The insulin-related hormones regulate key life processes in Metazoa, from metabolism to growth, lifespan and aging, through an evolutionarily conserved insulin signalling axis (IIS). The dmIR primary structure, with ~33% sequence identity in the overlapping regions, suggests that its domain organisation is similar to human IR-like receptors. dmIR domain topology, similar to hIR, is made of unique (αβ)2 subunit homodimers, with the same modular, exons-reflecting organisation. We selected the Drosophila DILP5 for dmIR-ECD studies as a typical representative and well-characterised fly ILP, having also a high homology to human insulin (~28% sequence identity), and with nM-range KD for the dmIR high-affinity site 1 of 0.76 (±0.16) nM21 that is within a range of human insulin:hIR interaction (e.g., 0.2–0.7 nM). Here, we provide the 3-D description of an invertebrate IR-like receptor by determining the cryoEM structure of the dmIR-ECD in the complex with DILP5.

The 5:1 molar hormone:receptor ratio used for the preparation of the dmIR-ECD complex resulted in an asymmetric three-DILP5:dmIR-ECD arrangement. There are two adjacent insulins bound to sites 1 and 2’ on the down-arm/dynamic and static protomers, respectively, and one insulin at site 1’ on the arm-up/static protomer. The overall DILP5’s binding modes in site 1 (down-arm (Λ) and up-arm site 1’ (Γ)) follows closely engagements of human insulins in respective h(m)IR sites. However, the third DILP5 molecule binds to site 2’ on the FnIII-1’ domain of the static protomer being adjacent to - and in contacts with - the down-arm site 1-bound DILP5, while site 2 is unoccupied. However, DILP5 sits ~6 Å lower on the FnIII-1’ side-surface than insulin in hIR’s sites 2/2’, with its B-helix also closer by ~2.7 Å to the FnIII-1’, especially when compared at the Cα atoms of ValB16(LeuB17) (in brackets: corresponding sequences of hIR (or human insulin)). This lowering of site 2’ DILP5 is likely required for the simultaneous accommodation of both DILP5s in sites 1 and 2’ in the lower-arm environment. Here, the shorter Lys884-Gly886 FnIII-1 loop minimises the steric hindrance upon binding of both DILP5s into the lower arm site1/2’ space, while the longer – dmIR specific - Ala1168-Ser1189 loop (with central short Ile1173-Thr1181 helix) provides a supporting ledge for the site 2’-bound hormone. In the dmIR-ECD this loop is slightly longer, and—importantly—it is reconfigured into a narrow β-hairpin that points directly into the DILP5 binding cavity that would be occupied by the C-domain of single-chain insulin-like family of hormones. Another characteristic structural feature of the dmIR-ECD is the reshaped - and slightly longer than in the hIR - Ala594-615Asn (Cys259-280His) CR-domain loop, which may prevent binding of any insulin-like hormone with a significant C-domain (e.g., hIGF-1-like).

>[2x]MHNYSYSPGISLLLFILLANTLAIQAVVLPAHQQHLLHNDIADGLDKTALSVSGTQSRWTRSESNPTMRLSQNVKPCKSMDIRNMVSHFNQLENCTVIEGFLLIDLINDASPLNRSFPKLTEVTDYIIIYRVTGLHSLSKIFPNLSVIRGNKLFDGYALVVYSNFDLMDLGLHKLRSITRGGVRIEKNHKLCYDRTIDWLEILAENETQLVVLTENGKEKECRLSKCPGEIRIEEGHDTTAIEGELNASCQLHNNRRLCWNSKLCQTKCPEKCRNNCIDEHTCCSQDCLGGCVIDKNGNESCISCRNVSFNNICMDSCPKGYYQFDSRCVTANECITLTKFETNSVYSGIPYNGQCITHCPTGYQKSENKRMCEPCPGGKCDKECSSGLIDSLERAREFHGCTIITGTEPLTISIKRESGAHVMDELKYGLAAVHKIQSSLMVHLTYGLKSLKFFQSLTEISGDPPMDADKYALYVLDNRDLDELWGPNQTVFIRKGGVFFHFNPKLCVSTINQLLPMLASKPKFFEKSDVGADSNGNRGSCGTAVLNVTLQSVGANSAMLNVTTKVEIGEPQKPSNATIVFKDPRAFIGFVFYHMIDPYGNSTKSSDDPCDDRWKVSSPEKSGVMVLSNLIPYTNYSYYVRTMAISSELTNAESDVKNFRTNPGRPSKVTEVVATAISDSKINVTWSYLDKPYGVLTRYFIKAKLINRPTRNNNRDYCTEPLVKAMENDLPATTPTKKISDPLAGDCKCVEGSKKTSSQEYDDRKVQAGMEFENALQNFIFVPNIRKSKNGSSDKSDGAEGAALDSNAIPNGGATNPSRRRRDVALEPELDDVEGSVLLRHVRSITDDTDAFFEKDDENTYKDEEDLSSNKQFYEVFAKELPPNQTHFVFEKLRHFTRYAIFVVACREEIPSEKLRDTSFKKSLCSDYDTVFQTTKRKKFADIVMDLKVDLEHANNTESPVRVRWTPPVDPNGEIVTYEVAYKLQKPDQVEEKKCIPAADFNQTAGYLIKLNEGLYSFRVRANSIAGYGDFTEVEHIKVEPPPSYAKDEVLFQGPSRSAWSHPQFEK;>DFRGVVDSCCRNSCSFSTLRAYCDS[3x];>NSLRACGPALMDMLRVACPNGFNSMFAK[3x]>[2x]MVKLFSFLLLVWVASPAFSSEFLKASGSNFYYGGQKVFLSGVNFAWRSYGSDFGNGQYASNGPALKDWINKVKASGGNTARVWVHVEGQVSPAFDSHGFVTSTDSKKTLINDLSDLLDYANGQNV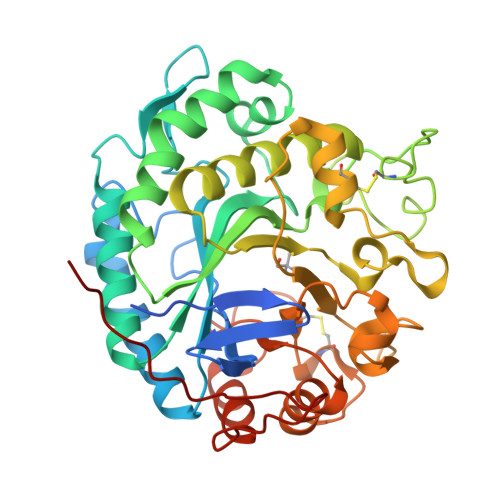FLILVLFNGALQNNSNVQNLFWDESKLNSYINNALTPMVNALKSKPSLAAWEVLNEPEGTLQPGSDQNSCYDTSTLAAQGAGWGGKKFPMKQILKTINWISSAIHNADSKALVTVGSWSELTQTDSFGYRNHYKDSCLTGAGGKSNGIINFYQMHTYSHSGKWNQNAPFKVNRWAYNVNDKPLLIGEFASVCSQNEGIQNLYKYAYNNGYNGALTWQFNSGGDCSDTYSNQMYGMQALKGQNDQSGGKGGMVSVNINHHHHHH>[4x]GSSHHHHHHMIDFGTIATAMVTPFDINGNIDFAKTTKLVNYLIDNGTTAIVVGGTTGESPTLTSEEKVALYRHVVSVVDKRVPVIAGTGSNNTHASIDLTKKATEVGVDAVMLVAPYYNKPSQEGMYQHFKAIAESTPLPVMLYNVPGRSIVQISVDTVVRLSEIENIVAIKDAGGDVLTMTEIIEKTADDFAVYSGDDGLTLPAMAVGAKGIVSVASHVIGNEMQEMIAAFQAGEFK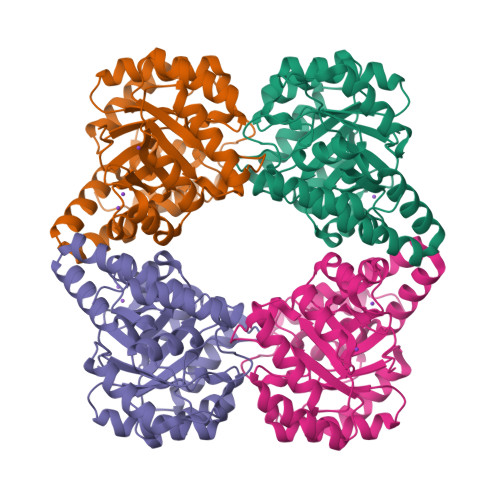KAQKLHQLLVRVTDSLFMAPSPTPVKTALQMVGLDVGSVRLPLLPLTEEERVTLQSVMQSIPR> GSSGSSGQFEVLERHTQWGLDLLDRYVKFVKERTEVEQAYAKQLRSLVKKYL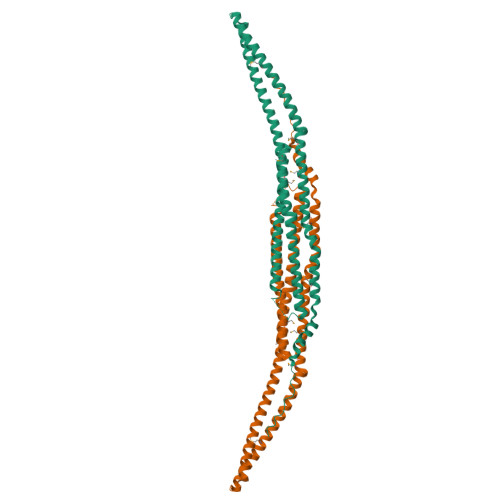PKRPAKDDPESKFSQQQSFVQILQEVNDFAGQRELVAENLSVRVCLELTKYSQEMKQERKMHFQEGRRAQQQLENGFKQLENSKRKFERDCREAEKAAQTAERLDQDINATKADVEKAKQQAHLRSHMAEESKNEYAAQLQRFNRDQAHFYFSQMPQIFDKLQDMDERRATRLGAGYGLLSEAELEVVPIIAKCLEGMKVAANAVDPKNDSHVLIELHKSGFARPGDVEFEDFSQPMNRAPSDSSLGTP> MTENILRKSDEEIQKEITARVKALESMLIEQGILTTSMIDRMAEIYENEVGPHL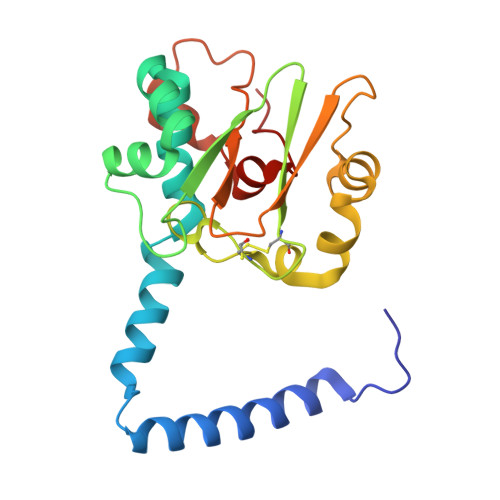GAKVVVKAWTDPEFKKRLLADGTEACKELGIGGLQGEDMMWVENTDEVHHVVVCTLCACYPWPVLGLPPNWFKEPQYRSRVVREPRQLLKEEFGFEVPPSKEIKVWDSSSEMRFVVLPQRPAGTDGWSEEELATLVTRESMIGVEPAKAV>AGAGAAGUUCUUCUCU[2x]

2-Thiouridine (s2U) is a nucleobase modification that confers enhanced efficiency and fidelity both on modern tRNA codon translation and on nonenzymatic and ribozyme-catalyzed RNA copying. We have discovered an unusual base pair between two 2-thiouridines that stabilizes an RNA duplex to a degree that is comparable to that of a native A:U base pair. High-resolution crystal structures indicate similar base-pairing geometry and stacking interactions in duplexes containing s2U:s2U compared to those with U:U pairs. Notably, the C=O···H–N hydrogen bond in the U:U pair is replaced with a C=S···H–N hydrogen bond in the s2U:s2U base pair.

We also designed an RNA sequence, UU2, that forms a duplex with two adjacent U:U pairs, 5′-AGA GAA GUUC UUC UCU-3′, as well as its thiolated analog, SS2, 5′-AGA GAA Gs2Us2UC UUC UCU-3′. However, SS2 exhibits a different packing with two strands forming a duplex in one asymmetric unit. While the SS1 and UU1 RNAs form very similar structures, the crystal packing of SS2, which contains two adjacent s2U:s2U base pairs, is slightly different from that of native UU2. In SS2, because there are two strands in one asymmetric unit, the two s2U:s2U base pairs are not identical, with two hydrogen bonds forming between different pairs of atoms. In the pair s2U9:s2U8′, the two hydrogen bonds are similar to those of the U:U pair in UU2, with one between the N3 of s2U8′ and O4 of s2U9, and another between S2 of s2U8′ and N3 of s2U9 (2.9 and 3.3 Å). However, the two hydrogen bonds in the pair s2U8:s2U9′ are between the O4 of s2U8 and N3 of s2U9′ and between N3 of s2U8 and S2 of s2U9′ (2.8 and 3.4 Å). Additionally, the distances between the two-position atoms (O or S) are longer in SS2 compared to UU2, which provides more room for each sulfur atom in SS2. For instance, the opening of the s2U:s2U pairs (−4.81°/–1.48°) is much smaller than that of the native U:U pairs (12.83°). The twist on the G7–U8/U9′–C10′ step on SS2 is less than that on UU2 (25.67 vs 42.98°) to provide a suitable angle to form the different hydrogen bonds on the s2U8:s2U9′ pair. As a result, the overlap area of G7-U8/U9′-C10′ is much smaller in SS2 than that in UU2 (3.86 vs 11.04 Å2), indicating a weaker base stacking interaction. These observations suggest that at least in our crystal structures both the hydrogen bonding and base stacking interactions in SS2 are weaker than those in UU2.>[2x]MKEVIAVKEITRFK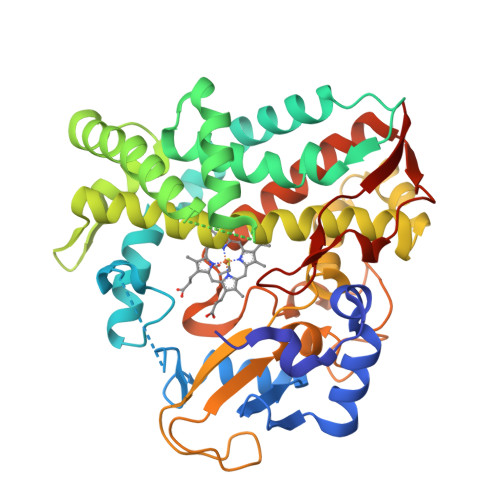TRTEEFSPYAWCKRMLENDPVSYHEGTDTWNVFKYEDVKRVLSDYKHFSSVRKRTTISVGTDSEEGSVPEKIQITESDPPDHRKRRSLLAAAFTPRSLQNWEPRIQEIADELIGQMDGGTEIDIVASLASPLPIIVMADLMGVPSKDRLLFKKWVDTLFLPFDREKQEEVDKLKQVAAKEYYQYLYPIVVQKRLNPADDIISDLLKSEVDGEMFTDDEVVRTTMLILGAGVETTSHLLANSFYSLLYDDKEVYQELHENLDLVPQAVEEMLRFRFNLIKLDRTVKEDNDLLGVELKEGDSVVVWMSAANMDEEMFEDPFTLNIHRPNNKKHLTFGNGPHFCLGAPLARLEAKIALTAFLKKFKHIEAVPSFQLEENLTDSATGQTLTSLPLKASRM> GSAVVALTNDRDTSYFGEIGIGTPPQKFTVIFDTGSSVLWVPSSKCINSKACRAHSMYESSDSSTYKENGTFGAIIYGTGSITGFFSQDSVTIGDLVVKEQDFIEATDEADNVFLHRLFDGILGLSFQTISVPVWYNMLNQGLVKERRFSFWLNRNVDEEEGGELVFGGLDPNHFRGDHTYVPVTYQYYWQFGIGDVLIGDKSTGFCAPGCQAFADSGTSLLSGPTAIVTQINHAIGA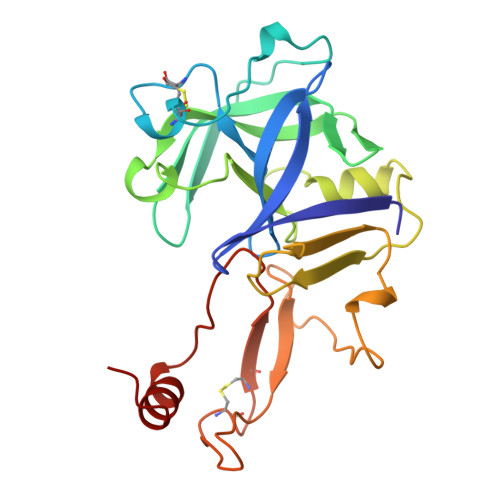N Ljungan virus (LV), a picornavirus originally isolated from voles, has been proposed as a zoonotic virus, potentially associated with type-1 diabetes mellitus, myocarditis and Guillain–Barré syndrome in humans. LV belongs to the Parechovirus genus and is closely related to human parechoviruses (HPeV) (∼48% amino-acid identity between the VP0 proteins). The capsid proteins (VP0, VP1 and VP3) adopt the expected eight-stranded anti-parallel β-barrel configuration and are arranged with pseudo T=3 symmetry (where T is the triangulation number), such that VP1 surrounds the five-fold axes and VP0 and VP3 alternate about the two- and three-fold axes. Structural comparisons place the virus close to HAV within the evolutionary hierarchy of picornaviruses, while substantial differences on both the inner and outer capsid surfaces, including the visualization of 12% of the RNA genome forming icosahedrally ordered interactions with the capsid, suggest the use of a charge-driven mechanism for genome encapsidation.

Here we report the determination of an atomic model of LV from a 3.78-Å resolution cryo-EM analysis. The LV capsid proteins are mostly well ordered, apart from residues 1–30 of VP1, 1–36 of VP0 and 1–3 of VP3. There are very marked (∼20 Å high) protrusions displaced some 45 Å from the icosahedral five-fold axes, but otherwise the external surface is broadly similar to that of other picornaviruses; being relatively smooth it is most similar to HAV21, although less angular. LV VP1 most closely resembles that of HAV, which likewise does not have a pocket factor (root mean squared deviation for 83% of Cαs is 2.0 Å); similar characteristics between the two viruses in VP1 are: a lengthened βH strand and alternative conformation of the GH loop blocking the entrance to the pocket, while the βC, βE, βF and βH strands shift so that it can no longer accommodate a lipidic pocket factor. LV uses the VP2 N-terminal domain swap across the icosahedral two-fold axis, first observed in a picornavirus for HAV21 (and seen in the insect picorna-like viruses), possibly imparting extra stability at this interface. The external surface of the LV capsid possesses unusual protrusions surrounding the five-fold axes, which extend the radius of the LV particle to ∼170 Å. Although these are poorly ordered and best seen in lower-resolution reconstructions, it is unambiguous that they are formed from the C terminus of VP1. Residues including Arg 6, Lys 7, Lys 9, Lys 12, Lys 14, Arg 49, Arg 62, Lys 64 of VP3 and Arg 225 of VP1 are engaged in interactions with the ordered RNA; of these, most of the VP3 residues are conserved across the genus, while residue 225 of VP1 is strictly conserved. Throughout the capsid the ordered RNA comprises some 900 bases, 12% of the viral genome. For other genera of the family, only occasional isolated bases have been observed.

> GLHSWGSEMDLVDSLDNPDEIQDNEEIQTQNVEAAQGEELATEVGLRATENDGSLSEQLNMSQPMFLNFKKHKVNIYAATHTKVDHIFGRAWAVGVFNTETAAIQKFDLHFPTSTHGALSRFFCHWTGELNIHILNVSTTNAFLKVAHTWFGTDSGIARTATLESNGTMIIPPNEQMTLCVPYYSEVPLRCVKGSDRNSAGLGSLFTQAVGRTISNRVQIFVSFRCPNFFFPLPAPREATSASILERVDEANAEELEAVLEARTPDAPLRLKFNPEDPLKQLREAAKAYFNIMHSDE;> MAASKMNPVGNLLSTVSSTVGSLLQNPSVEEKEMDSDRVAASTTTNAGNLVQASVAPTMPVKPDFKNTDDFLSMSYRSTTAPTNPTKMVHLAHGTWTTNQHRQALVASITLLQAFWPNQDFPAWGQSRYFAAVRCGFHIQVQLNVNIGSAGCLIAAYMPKTAHDHMNTYTFGSYTNLPHVLMNAATTSQADLYIPYVFNHNYARTDSDDLGGIYIWVWSALTVPSGSPTTVDVTIFGSLLDLDFQCPRPPGADTVIYTQ;> GKRTVRKTKTSKFKWVRNKIDIAEGPGAMNIANVLSTTGGQTIALVGERAFYDPRTAGAAVRCKDLMEIARMPSVFLGESTEPDGRRGYFTWSHTISPVNWVFDDHIYLENMPNLRLFSSCYNYWRGSFVIKLTVYASTFNKGRLRMAFFPNREGAYTQDDAQNAIFVVCDIGLNNTFEMTIPYTWGNWMRPTRGNSLGHLRIDVLNRLTYNSSSPNAVNCILQIKMGDDAMFMVPTTSNLVMQ> SLSWDSVVERIRIFLVESPIKMARLQGVGNVKGSVKRVLLEVTSADGIVGWGEAAPWEVFTGTPEAAFSALDIYLRPLILGAPIKRVRELMARMDKMLVGHGEAKAAVEMALLDILGKATGLSVADLLGGRVRDRIPLSFSIADPDFDADLERMRAMVPAGHTVFKMKTGVKPHAEELRILETMRGEFGERIDLRLDFNQALTPFGAMKILRDVDAFRPTFIEQPVPRRHLDAMAGFAAALDTPILADESCFDAVDLMEVVRRQAADAISVKIMKCGGLMKAQSLMAIADTAGLPGYGGTLWEGGIALAAGTQLIAATPGISLGCEFYMPHHVLTEDVLEERIANSAGHVIVPDGPGLGISISEAS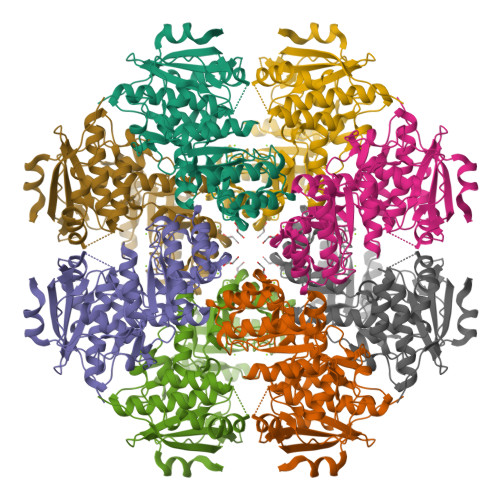LRGNAKILAER> MTSFTIPGLSDKKASDVADLLQKQLSTYNDLHLTLKHVHWNVVGPNFIGVHEMIDPQVELVRGYADEVAERIATLGKSPKGTPGAIIKDRTWDDYSVERDTVQAHLAALDLVYNGVIEDTRKSIEKLEDLDLVSQDLLIAHAGELEKFQWFVRAHLESAGGQLTHEGQSTEKGAADKARR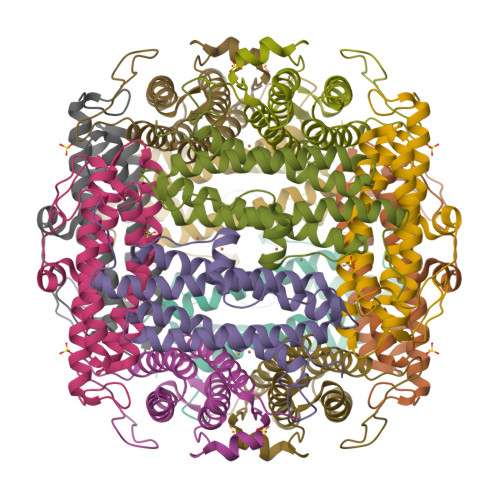KSA>DPSSRSTRKAVIGYYFIPTNQINNYTETDTSVVPFPVSNITPAKAKQLTHINFSFLDINSNLECAWDPATNDAKARDVVNRLTALKAHNPSLRIMFSIGGWYYSNDLGVSHANYVNAVKTPASRAKFAQSCVRIMKDYGFDGVDIDWEYPQAAEVDGFIAALQEIRTLLNQQTITDGRQALPYQLTIAGAGGAFFLSRYYSKLAQIVAPLDYINLMTYDLAGPWEKVTNHQAALFGDAAGPTFYNALREANLGWSWEELTRAFPSPFSLTVDAAVQQHLMMEGVPSAKIVMGVPFYGRAFKGVSGGNGGQYSSHSTPGEDPYPSTDYWLVGCEECVRDKDPRIASYRQLEQMLQGNYGYQRLWNDKT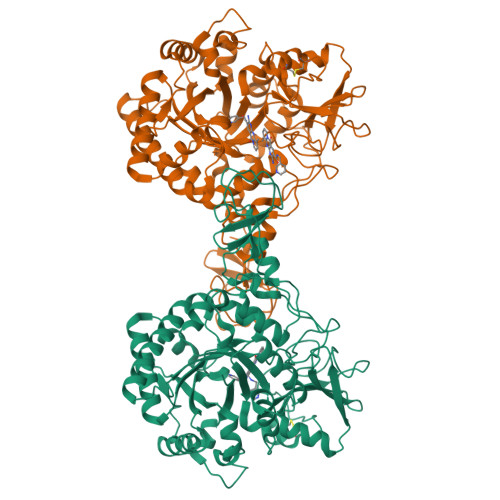KTPYLYHAQNGLFVTYDDAESFKYKAKYIKQQQLGGVMFWHLGQDNRNGDLLAALDRYFNAADYDDSQLDMGTGLRYTGVGPGNLPIMTAPAYVPGTTYAQGALVSYQGYVWQTKWGYITSAPGSDSAWLKVGRVAHHHHHH[2x]> GSNRRLQQTQAQVDEVVDIMRVNVDKVLERDQKLSELDDRADALQAGASQFETSAAKLKRKYW;> GSALSE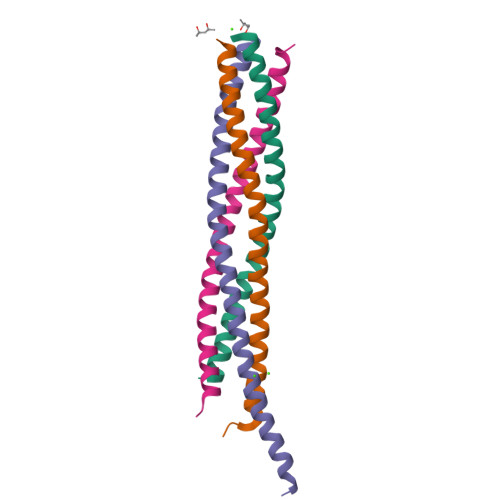IETRHSEIIKLENSIRELHDMFMDMAMLVESQGEMIDRIEYNVEHAVDYVERAVSDTKKAVK;> GSMRNELEEMQRRADQLADESLESTRRMLQLVEESKDAGIRTLVMLDEQGEQLDRVEEGMNHINQDMKEAEKNLKDLGK;> GSARENEMDENLEQVSGIIGNLRHMALDMGNEIDTQNRQIDRIMEKADSNKTRIDEANQRATKMLG> MDELVKALERAGYLLTPSAYYLLVDHFKEGKFSLVELVKFAKSKGVFIIDGDLAYEFLQFLGLGVPQEIKESYISTGEEAEKTVESQETRASELEEGGVSQVSSGELQELKEESPEISTTEEEIGGLELVQSSISTGSEVEYNNGENGESVVVLDKYGYPILYAPEEIGEEKEYSKYEDVVIEWNPSVTPVQIEKNYEVKFDVRQVKLRPPKVKNGSGKEGEIIVEAYASLFKSRLSKLKRILRENPEISNVVDIGKLNYVSGDEEVTI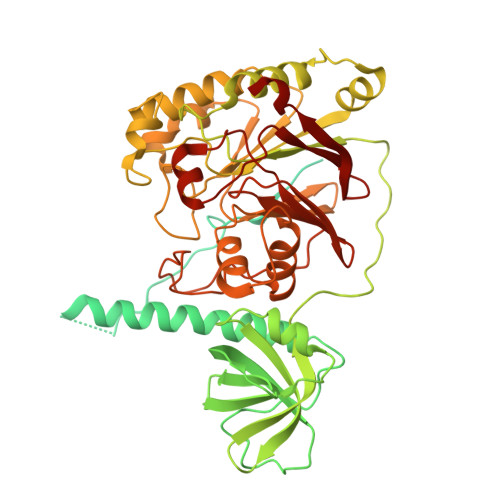IGLVNSKRETNRGLIFEVEDKTGIVKVFLPKDSEDYREAFKVLPDAVVAFKGFYSKKGIFFANKFYLPDVPLYRKQKPPLEEKVYAILISDIHVGSREFCEKAFLKFLEWLNGHVESKEEEEIVSRVKYLIIAGDVVDGIGIYPGQYSDLVIPDIFDQYEALANLLANVPEHITMFIGPGNADAARPAIPQPEFYKEYAKPIYKLKNAIIISNPAVIRLHGRDFLIAHGRGIEDVVSFVPGLTHHKPGLPMVELLKMRHLAPTFGGKVPIAPDPEDLLVIEEVPDLVQMGHVHVYDAVVYRGVQLVNSATWQAQTEFQKMVNIVPTPAKVPVVDVESARVVKVLDFSGWC(1R,2S)-1-hydroxybutane-1,2,4-tricarboxylic 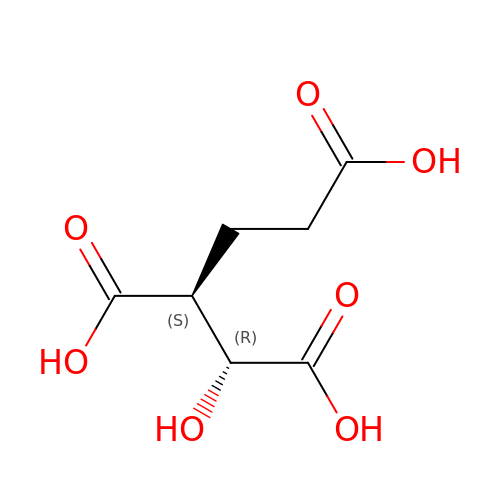acid | C7 H10 O7 | OEJZZCGRGVFWHK-WVZVXSGGSA-N>[2x]ASQNSFRIEYDTFGELKVPNDKYYGAQTVRSTMNFKIGGVTERMPTPVIKAFGILKRAAAEVNQDYGLDPKIANAIMKAADEVAEGKLNDHFPLVVWQTGSGTQTNMNVNEVISNRAIEMLGGELGSKIPVHPNDHVNKSQSSNDTFPTAMHIAAAIEVHEVLLPGLQKLHDALDAKSKEFAQIIKIGRTHTQDAVPLTLGQEFSGYVQQVKYAMTRIK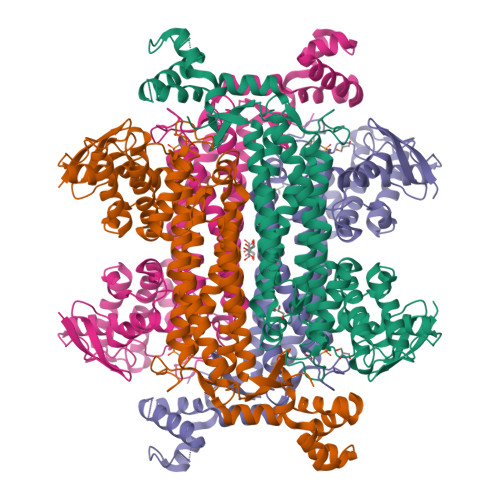AAMPRIYELAAGGTAVGTGLNTRIGFAEKVAAKVAALTGLPFVTAPNKFEALAAHDALVELSGAMNTTACSLMKIANDIRFLGSGPRSGLGELILPENEPGSSIMPGKVNPTQCEAMTMVAAQVMGNHVAVTVGGSNGHFELNVFKPMMIKNVLHSARLLGDASVSFTENCVVGIQANTERINKLMNESLMLVTALNPHIGYDKAAKIAKTAHKNGSTLKETAIELGYLTAEQFDEWVKPKDMLGPK CYANIDE ION | C N | 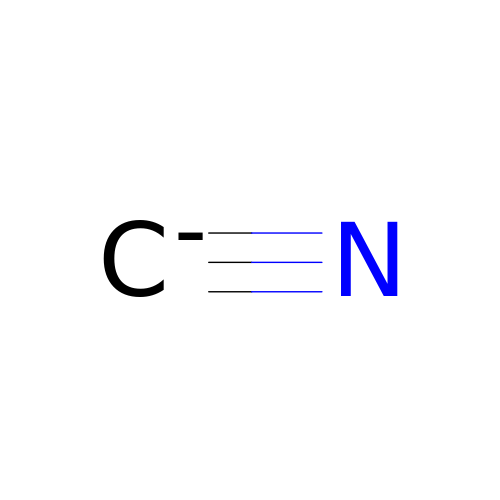XFXPMWWXUTWYJX-UHFFFAOYSA-N> QPIFLNVLEAIEPGVVCAGHDNNQPDSFAALLSSLNELGERQLVHVVKWAKALPGFRNLHVDDQMAVIQYSWMGLMVFAMGWRSFTNVNSAMLYFAPDLVFNEYRMHKSRMYSQCVRMRHLSQEFGWLQITPQEFLCMKALLLFSIIPVDGLKNQKFFDELRMNYIKELDRIIACKRKNPTSCSRRFYQLTKLLDSVQPIAR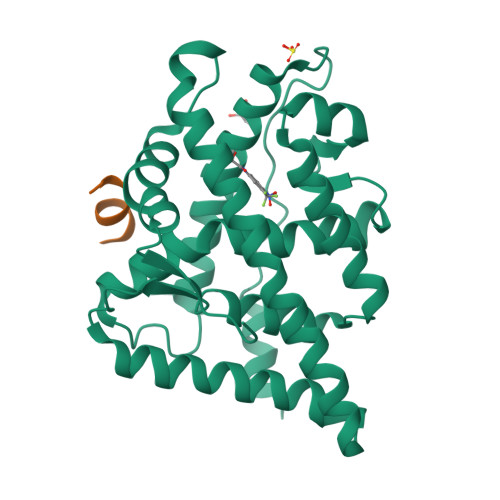ELHQFAFDLLIKSHMVSVDFPEMMAEIISVQVPKILSGKVKPIYFHTQ;> SDSAFSRYYTRS Using Arabidopsis thaliana Pdx1, an enzyme involved in vitamin B6 biosynthesis, and lysozyme, we demonstrate crystal scaling to suitable dimensions and numbers for time-resolved serial crystallography. Here, we report the use of droplet miniaturization for the controlled production of uniform crystals, providing an avenue for controlled substrate addition and synchronous reaction initiation. The approach was evaluated using two enzymatic systems, yielding 3 µm crystals of lysozyme and 2 µm crystals of Pdx1, an Arabidopsis enzyme involved in vitamin B6 biosynthesis. The method was demonstrated with lysozyme and Pdx1, with crystals grown in droplets producing equivalent (if not better) diffraction data quality to those produced under batch conditions.

Crystals for preparing seeds were produced by combining (1:1) ∼12 mg ml−1 Pdx1 with mother liquor (600 mM sodium citrate, 100 mM HEPES pH 7) as 10 µl vapour diffusion drops in 24-well XRL plates (Molecular Dimensions). Crystals for seed stocks grew overnight and varied in size from 10 to 50 µm in length. Vortexing with a Hampton Seed Bead was carried out for a total of 180 s by alternating between 30 s of vortexing and 30 s on ice followed by storage at −20°C. Batch crystallization involved a 1:1:1 mixture of 12 mg ml−1 Pdx1, seed (105–107 ml−1) and mother liquor. A popular strategy is to fragment crystals to make seeds to control crystal growth. Seeds effectively bypass nucleation, acting as nuclei to instantly initiate growth such that protein is shared throughout crystal growth. Lysozyme and Pdx1 crystals were concentrated by settling and applied to sheet-on-sheet (SOS) chips. Serial synchrotron crystallography (SSX) data for lysozyme and Pdx1 crystals grown in batch and within microfluidic droplets were collected on the new ID29 beamline at the European Synchrotron Radiation Facility (ESRF, France) using a 2 × 4 µm (V × H) beam of 11.56 keV X-rays, with a 90 µs pulse and 231.25 Hz repetition rate, and a 20 µm step movement between images. A JUNGFRAU 4M detector with a sample-to-detector distance of 175 mm (1.8 Å in the corner) was used to collect diffraction patterns.

>MEGTGVVAVYGNGAITEAKKSPFSVKVGLAQMLRGGVIMDVVNAEQARIAEEAGACAVMALERVPADIRAQGGVARMSDPQMIKEIKQAVTIPVMAKARIGHFVEAQILEAIGIDYIDESEVLTLADEDHHINKHNFRIPFVCGCRNLGEALRRIREGAAMIRTKGEAGTGNIIEAVRHVRSVNGDIRVLRNMDDDEVFTFAKKLAAPYDLVMQTKQLGRLPVVQFAAGGVATPADAALMMQLGCDGVFVGSGIFKSGDPARRARAIVQAVTHYSDPEMLVEVSCGLGEAM[4x]> MQTFLIMYAPMVVVALSVV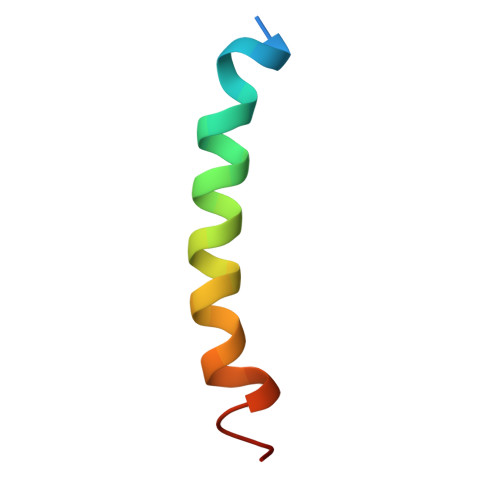AAFWVGLKDVHVNE> EEDDEFEDFPIDTWANGETIKSNAVTQTNIWEENWDDVEVD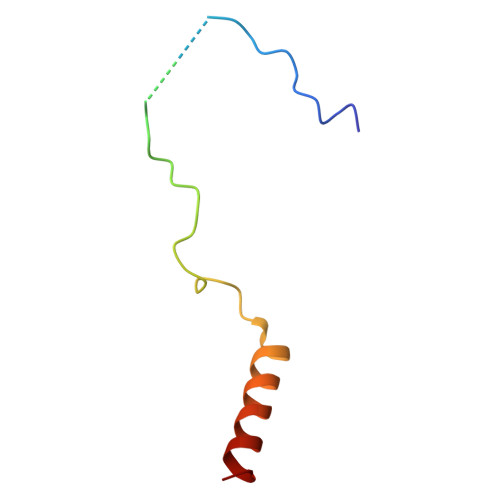DDFTNELKAELDRYKRENQ1-DEOXY-1-(8-IODO-7-METHYL-2,4-DIOXO-3,4-DIHYDROBENZO[G]PTERIDIN-10(2H)-YL)-D-RIBITOL 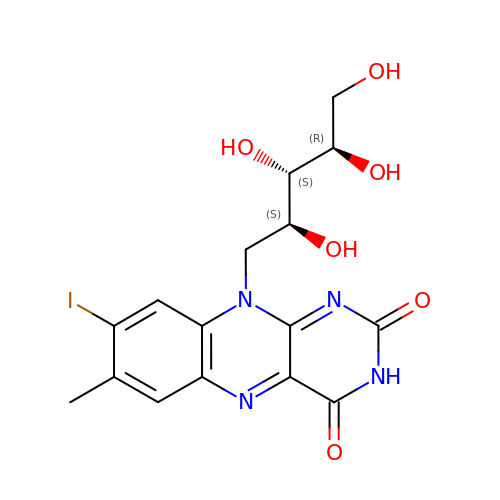| C16 H17 I N4 O6 | GXUZMSUHTJJUNU-LOWVWBTDSA-N> MKLSPREVEKLGLHNAGYLAQKRLARGVRLNYTEAVALIASQIMEYARDGEKTVAQLMCLGQHLLGRRQVLPAVPHLLNAVQVEATFPDGTKLVTVHDPISRENGELQEALFGSLLPVPSLDKFAETKEDNRIPGEILCEDECLTLNIGRKAVILKVTSKGDRPIQVGSHYHFIEVNPYLTFDRRKAYGMRLNIAAGTAVRFEPGDCKSVTLVSIEGNKVIRGGNAIADGPVNETNLEAAMHAVRSKGFGHEEEKDASEGFTKEDPNCPFNTFIHRKEYANKYGPTTGDKIRLGDTNLLAEIEKDYALYGDECVFGGGKVIRDGMGQSCGHPPAISLDTVITNAVIIDYTGIIKADIGIKDGLIASI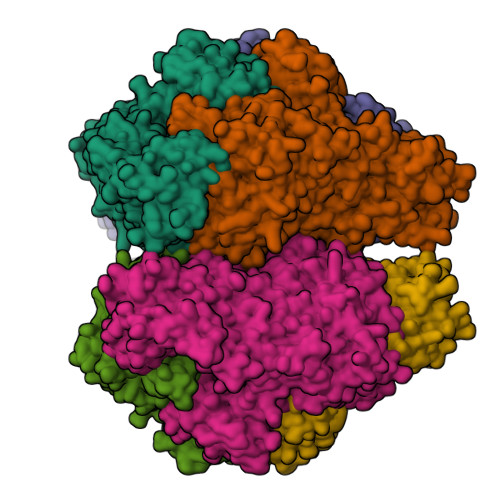GKAGNPDIMNGVFSNMIIGANTEVIAGEGLIVTAGAIDCHVHYICPQLVYEAISSGITTLVGGGTGPAAGTRATTCTPSPTQMRLMLQSTDDLPLNFGFTGKGSSSKPDELHEIIKAGAMGLKLHEDWGSTPAAIDNCLTIAEHHDIQINIHTDTLNEAGFVEHSIAAFKGRTIHTYHSEGAGGGHAPDIIKVCGIKNVLPSSTNPTRPLTSNTIDEHLDMLMVCHHLDREIPEDLAFAHSRIRKKTIAAEDVLNDIGAISIISSDSQAMGRVGEVISRTWQTADKMKAQTGPLKCDSSDNDNFRIRRYIAKYTINPAIANGFSQYVGSVEVGKLADLVMWKPSFFGTKPEMVIKGGMVAWADIGDPNASIPTPEPVKMRPMYGTLGKAGGALSIAFVSKAALDQRVNVLYGLNKRVEAVSNVRKLTKLDMKLNDALPEITVDPESYTVKADGKLLCVSEATTVPLSRNYFLF> GSHMRKIQRYVRKDGKCNVHHGNVREKRAETLVFSTHAVISMRDGKLCLMFRVGDLRNSHIVEASIRAKLIK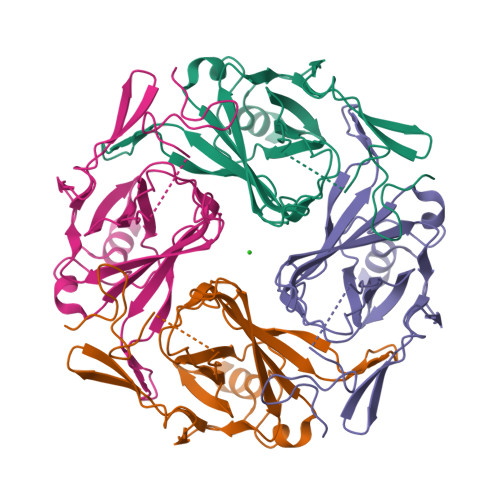SKQTSEGEFIPLNQTDINVGYYTGDDRLFLVSPLIISHEINQQSPFWEISKAQLPKEELEIVVILEGMVEATGMTCQARSSYITSEILWGYRFTPVLTLEDGFYEVDYNSFHETYETSTPSLSAKELAELANRAEL> MISLNGYGRFGLQYVEDRGVGLEDTIISSRLRINIVGT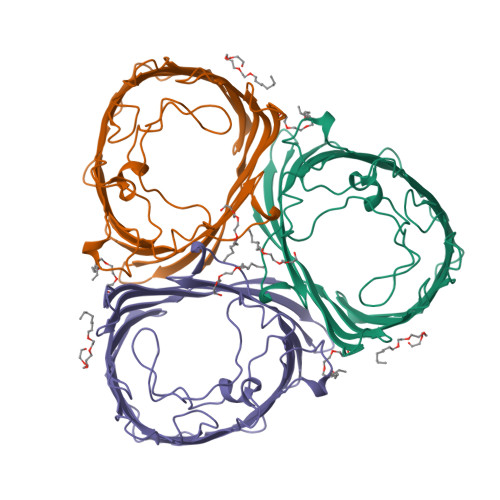TETDQGVTFGAALAMQWDDGDAFAGTAGNAAQFWTSYNGVTVSVGNVDTAFDSVALTYASAMGYEASSFGDAQSSFFAYNSKYDASGALDNYNGIAVTYSISGVNLYLSYVDPDQTVDSSLVTEEFGIAADWSNDMISLAAAYTTDAGGIVDNDIAFVGAAYKFNDAGTVGLNWYDNGLSTAGDQVTLYGNYAFGATTVRAYVSDIDRAGADTAYGIGADYQFAEGVKVSGSVQSGFANETVADVGVRFDF As the pentose phosphate pathway (PPP) is the main NADPH supplier in most parasites, the enzymes of this key metabolic pathway are considered promising drug targets for the control of unicellular parasites such as Leishmania, Trypanosoma and Plasmodium. Under native conditions, the SEC profiles of Ld6PGD wt revealed one stable peak representing a molecular mass of 94–111 kDa, which is equivalent to the dimeric form of the Ld6PGD wt and in accordance with previously published SEC profiles from Leishmania 6PGDs. Each subunit of the homodimer comprises a NADP+ and a 6PG binding site. The C-terminal tail of domain 2 (M438-Q478) invades the neighboring subunit so that each active site is built by residues of both subunits.

In addition, we solved the three-dimensional crystal structure of Ld6PGD in complex with NADP(H), revealing a previously unknown conformation of NADPH. The crystal contained two monomers in the asymmetric unit (AU), which were essentially similar to an RMSD of 0.4 Å (478 residues). The omit maps displayed clear density for one phosphate ion in each subunit and one NADP(H) molecule in subunit A. In subunit B, most of the NADP(H) molecule is well defined by electron density, except for the nicotinamide and the adenine moieties, which are not visible. In our Ld6PGD structure, NADP(H) is located at the conserved NADP+ binding site. The amino acids N31, R32 and T33 interact with one of the phosphates, N31 and N104 with the ribose moieties and the diphosphates are bound by main chain atoms of residues V11 and M12. Via van der Waals forces, I129 and S130 interact with the nicotinamide ring, which is also hydrogen bonded to a phosphate ion. According to this, the active site loop residues (D257-T262) of the Ld6PGD structure, complexed with a phosphate at the 6PG binding site, adopt the closed conformation. Since Ld6PGD was crystallized under catalysis, in the presence of both substrates, 6PG and NADP+, it could be also the products (R5P, NADPH) or an intermediate state of substrate and product that are visible in the active site. Since crystallization with an excess of 6PG and NADP+ in the crystallization buffer, and thus under catalysis, could have resulted in a feedback inhibition by high concentrations of the product NADPH, we suggest that Ld6PGD is complexed with NADPH in its inhibitory conformation, in which the nicotinamide ring occupies part of the 6PG binding site. As the nicotinamide ring occupies part of the 6PG binding pocket, we hypothesize that only the phosphate component of 6PG can bind at the usual site, while the rest of the 6PG molecule must be flexible and therefore not visible in the electron density.

>[2x]SNDLGIIGLGVMGANLALNIAEKGFKVAVFNRTSAKTASFLKEHESEKFAANLNGYETMKAFAASLKKPRRAFILVQAGAATDSTIEQLKEVLENGDIIIDTGNANFKDQDKRAAQLESQGLRFLGMGISGGEEGARKGPAFFPGGTPSVWEEVRPIVEAAAAKAEDGRPCVTFNGKGGAGSCVKMYHNAGEYAVLQIWGEAYTALLAFGFDNDQIADVFESWKADGFLKSYMLDISIAACRAREAAGNYLSEKVKDRIGSKGTGLWSAQEALEVGVPAPSLSMAVISRQMTMCKEERIANCKAFPNFPRGPSAEARDKSPNSPDAKQLYHAVSLCIIASYAQMFQCLRELDKVYGFGLNLPATIATFRAGCILQGYLLGPMTKAFEENPSLPNLMDAFTKEIVAGLDDCRQILAKLTVNTAVSLPVMMASLSYINAMYTETLPYGQLVSLQRDVFGRHGYERTDKDGRESFEWPALQ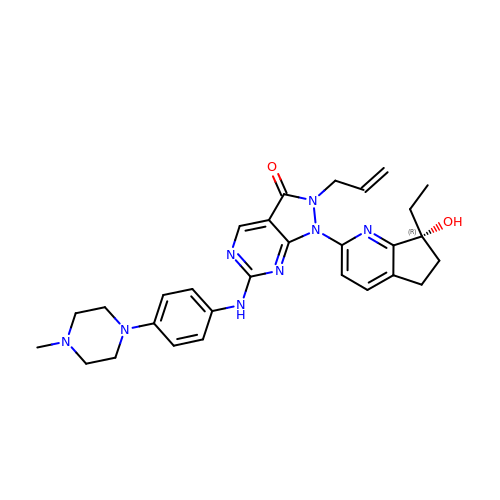1-[(7R)-7-ethyl-7-hydroxy-6,7-dihydro-5H-cyclopenta[b]pyridin-2-yl]-6-[4-(4-methylpiperazin-1-yl)anilino]-2-(prop-2-en-1-yl)-1,2-dihydro-3H-pyrazolo[3,4-d]pyrimidin-3-one | C29 H34 N8 O2 | OXTSYWDBUVRXFF-GDLZYMKVSA-N>GSEELLDLFNRQVTQEFTASQVYLSASIWFDQNDWEGMAAYMLAESAEEREHGLGFVDFANKRNIPIELQAVPAPVSCAEWSSPEDVWQSILELEQANTRSLLNLAEAASTCHDFAVMAFLNPFHLQQVNEEDKIGSILAKVTDENRTPGLLRSLDVVSFLGPCLFRS[6x]

A novel ferritin was recently found in Pseudo-nitzschia multiseries (PmFTN), a marine pennate diatom that plays a major role in global primary production and carbon sequestration into the deep ocean. Ferritin is a 24-mer that forms a hollow sphere, takes up soluble ferrous iron, oxidizes it at di-iron ferroxidase centers, and stores the iron oxide mineral in its central cavity. Sites A and B comprise the conserved ferroxidase active site, and site C forms a pathway leading toward the central cavity where iron storage occurs. The structures confirm the typical ferritin arrangement: 24 subunits assemble to form a hollow spherical shell.

To determine whether occupation of ferroxidase sites and site C is time-dependent, apo-PmFTN crystals were soaked for 5 min, 45 min, 4 h, and overnight in 2 mm ferrous sulfate. Structures of crystals exposed to ferrous iron for 4 h or longer revealed iron bound in all three sites as well as up to two additional sites at the inner surface of the ferritin sphere. The latter two sites may serve as the nucleation site for formation of the mineral core. All but one of the crystals analyzed were of space group P23 with eight ferritin monomers in the asymmetric unit. A bridging oxygen atom is modeled between sites A and B and between sites B and C. A second solvent oxygen atom is coordinated to iron in site A. The bridging solvent molecule between sites A and B might be a bridging oxo group rather than a water molecule, building a diferric-oxo bridge as seen in other ferritins. Sample electron density for the overnight-soaked structure at the ferroxidase site including the bridging ligand is presented in Fig. 2D. Glu-130 adopts multiple conformations depending on the soaking time and is observed coordinated to iron atoms in site B and/or site C. In the overnight-soaked structure, Glu-130 is tilted toward the iron in site B, whereas in the 4-h-soaked structure, it is predominately coordinated to site C. The distance between the iron atoms in sites A and B is ∼3.8 Å in Fe, which decreases to ∼3.6 Å upon overnight soak. In PmFTN, iron occupancy at both sites is only observed after prolonged iron exposure, and the site A and B intermetal distance of less than 3.8 Å decreases only slightly with time to 3.6 Å, suggesting that in the structures where iron is bound to both sites it is in the Fe(III) state.> WENTSYILGVDAKGKQERTDKCHAAFIAHIKAYCDTADQDLAAVLQFLEHGEKDLSAFPVSEEVIGSNIVFRIEGEPGFVHERPAARQAWANCLNRREQGLCGQCLITGERQKPIAQLHPSIKGGRDGVRGAQAVASIVSFNNTAFESYGKEQSINAPVSQEAAFSYVTALNYLLNPSNRQKVTIADATVVFWAERSSPAEDIFAGMFDPPSTTAKPESSNGTPPEDSEEGSQPDTARDDPHAAARMHDLLVAIRSGKRATDIMPDMDESVRFHVLGLSPNAARLSVRFWEVDTVGHMLDKVGRHYRELEIIPQFNNEQEFPSLSTLLRQTAVLNKTENISPVLAGGLFRAMLTGGPYPQSLLPAVLGRIRAEHARPEDKSRYRLEVVTYYRAALIKAYLIRNRKLEVPVSLDPARTDRPYLLGRLFAVLEKAQEDAVPGANATIKDRYLASASANPGQVFHMLLKNASNHT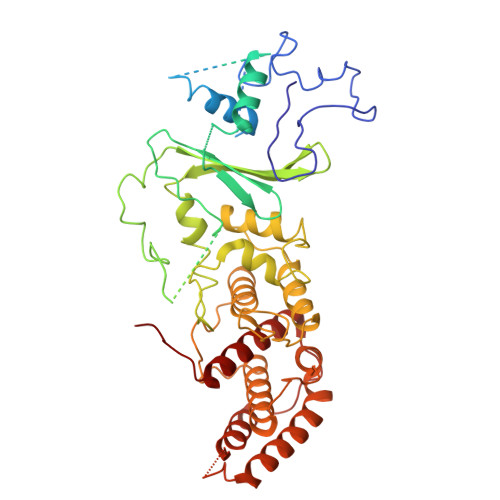AKLRKDPERKGSAIHYEIMMQEIIDNISDFPVTMSSDEQGLFMIGYYHQRKALFTKKNKEN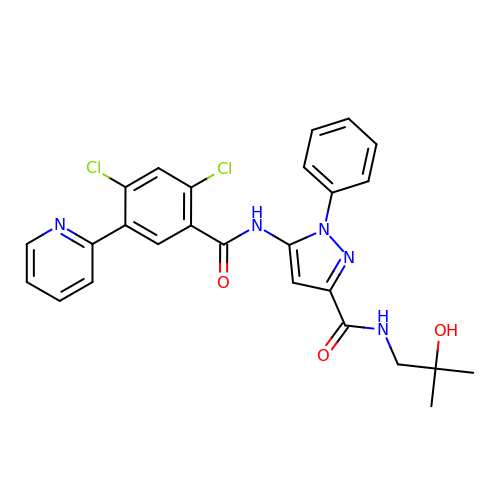5-{[2,4-dichloro-5-(pyridin-2-yl)benzene-1-carbonyl]amino}-N-(2-hydroxy-2-methylpropyl)-1-phenyl-1H-pyrazole-3-carboxamide | C26 H23 Cl2 N5 O3 | NXDRKVFQQJUBOG-UHFFFAOYSA-N>[2x]MKHPFSRLFSFGEKEQEEMEEKQEREEVRHIPVKSIIPNRFQPRTMFDEEKIDELALTIRTHGIIQPIVVRECGNGRFEIIAGERRWRAVQKLGWTEIPAIIKNLNDKETASVALIENLQREELTPIEEAMAYAKLIELHDLTQEALAQRLGKGQSTIANKLRLLKLPQEVQEALLQRAITERHARALIALKDKEKQLKLLQEIIDKQLNVKQTEDRVLKLLEAGERKPKPKRKAFSRDKLAAALEHH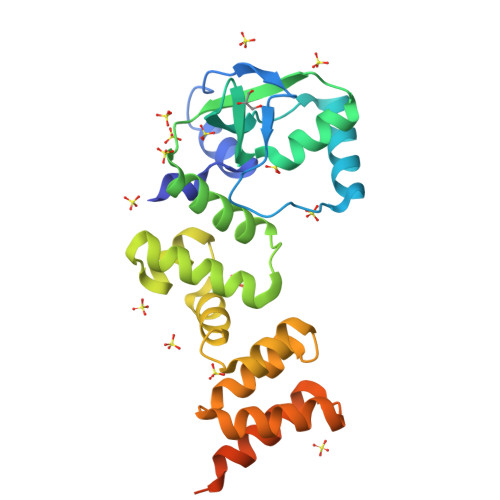HHHH>GSAAAQDMVSPPPPIADEPLTVNTGIYLIESYSLDDCAETFKVNAFLSLSWKDRRLAFDPVRSGVRVKTYEPEAIWIPEIRFVNVENARDADVVDISVSPDGTVQYLERFSARVLSPLDFRRYPFDSQTLHIYLIVRSVDTRNIVLAVDLEKVGKNDDVFLTGWDIESFTAVVKPANFALEDRLESKLDYQLRISRQYFSYIPNIILPMLFILFISWTAFWSTSYEANVTLVVSTLIAHIAFNILVETCLPKTPYMTYTGAIIFMIYLFYF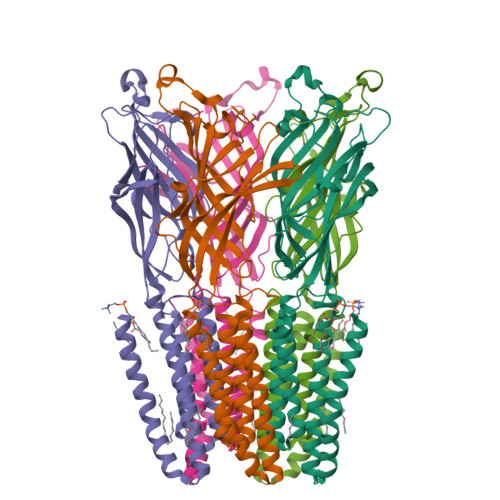VAVIEVTVQHYLKVESQPARAASITRASRIAFPVVFLLANIILAFLFFGF[10x]> MPTPSHLKNPLCFDFRAARRVPETHAWPGLDDHPVVDGGGGGGEDAVPVVDVGAGDAAARVARAAEQWGAFLLVGHGVPAALLSRVEERVARVFSLPASEKMRAVRGPGEPCGYGSPPISSFFSKLMWSEGYTFSPSSLRSELRRLWPKSGDDYLLFCDVMEEFHKEMRRLADELLRLFLRALGLTGEEVAGVEAERRIGERMTATVHLNWYPRCPEPRRALGLIAHTDSGFFTFVLQSLVPGLQLFRRGPDRWVAVPAVAGAFVVNVGDLFHILTNGRFHSVYHRAVVNRDRDRVSLGYFLGPPPDAEVAPLPEAVPAGRSPAYRAVTWPEYMAVRKKAFATGGSALKMVSTDAAAAADEHDDVAAAADVHA

GAs are synthesized in a stepwise manner by multiple oxidases, and the conversion from direct precursors to bioactive GAs is mediated by GA 3-oxidases (GA3oxs). GA3ox and GA2ox, members of the 2-oxoglutarate (2OG)- and Fe (II)-dependent dioxygenase (2ODD) family, catalyze the oxidation of substrate GAs using 2OG and molecular oxygen as co-substrates and ferrous Fe(II) cofactors. Rice harbors two GA3ox genes, which encode GA3-oxidases that catalyze the final step of GA biosynthesis, i.e., the addition of a hydroxyl group at C3 of GA precursors. Here, we report the functional and evolutionary analyses of rice gibberellin 3-oxidase 1 (OsGA3ox1), a gibberellin synthetic enzyme specifically expressed in the late developmental stages of anthers.

To understand why OsGA3ox1 produced higher levels of GA7 compared to OsGA3ox2, we performed X-ray crystallography analyses of these enzymes. As a result, we succeeded in obtaining the structure of the OsGA3ox2 complex with (co-) substrates; GA9 and 2-oxoglutarate (2OG) at 1.9 Å resolution. Fe (II) was eliminated for crystallization to prevent the enzyme reaction, as previously described. The carboxyl group of GA9 established interaction with S230, G231, F233, T234, and R337 directly or indirectly through water, and its γ-lactone ring established interaction with the main chain of I119. These amino acids are conserved between OsGA3ox1 and OsGA3ox2, but not between OsGA2oxs, OsGA20oxs, or even AtGA3oxs, with the exception that I119 is replaced with Y in OsGA3ox1. Moreover, upon comparing the structure of OsGA3ox2 with that of OsGA2ox3, we found that the GAs were inverted in the substrate-binding pocket. Conversely, the residues H227, D229, and H285 of OsGA3ox2 established interaction with Fe (II); Y212, S297, and R295 established interaction with 2OG. These amino acids are highly conserved in almost all 2ODDs, except F235 in OsGA3ox1, which is a conserved Y residue in other 2ODDs. Taken together, these results indicate that the substitution of a highly conserved Y with F in OsGA3ox1 contributes to the hyperproductivity of GA7. Whereas the main product of OsGA3ox2 was GA4 (OsGA3ox2), we found a remarkable peak of GA7 as well as GA4 when we analyzed OsGA3ox1 (OsGA3ox1).Compared to the RdRPs of other Flaviviridae representatives such as the NS5 of the Japanese encephalitis virus (JEV) and dengue virus (DENV) in the Flavivirus genus and the NS5B of the hepatitis C virus (HCV) of the Hepacivirus genus, the pestivirus NS5B contains a unique ∼90-residue N-terminal domain (NTD) that does not have notable sequence homology to any other viral or host proteins. The global conformation of our CSFV NS5B structures is consistent with the recently reported CSFV structure with an RMSD value of 0.9 Å (95% coverage) between the reported structure and our representative C-682 structure. These structures together reveal that the NTD adopts a globular α/β fold with an α-β-α-β-β-α pattern. The NTD interacts with the palm of the RdRP core intra-molecularly with a mixture of hydrophobic and hydrogen bonding interactions. Collectively, these biochemical data indicated that the RNA synthesis fidelity of CSFV NS5B is fine-tuned by its NTD through the intra-molecular interactions with the RdRP palm.

To better understand the nature of the NTD–RdRP intra-molecular interface interactions and whether they regulate the RdRP fidelity, we designed point mutations at the Y471 and E472 sites in the context of the WT NS5B and the N- and C-terminal deletion mutants. Crystallization screenings were performed for all the NTD containing mutant constructs and four of them were successfully crystallized with one construct crystallized under two different conditions. Among these five structures, three of them (Y471A and two forms of C-672_Y471A) maintain the WT conformation with the NTD–RdRP intra-molecular interface maintained. The NTD–RdRP intra-molecular interactions are fully disrupted, and the NTD is rather involved in a non-intensive three-way interaction involving two symmetry-related neighboring NS5B molecules in the crystal lattice. These structural data together suggest that the selection of Y471-E472 mutation sites is valid in perturbing the NTD–RdRP interface, but the interface may not necessarily be fully disrupted by some of the mutations. The effect of E472A mutation was highly consistent with AA mutation (compare lanes 4/8/14/18 to 5/9/15/19), while the effect of Y471A mutation was slightly smaller than that of the E472A and AA mutations (compare lanes 3/7/13/17 to 4/8/14/18 and 5/9/15/19). Although NTD–RdRP disengagement, a situation mimicked by the crystallographic open conformation state in a crystal lattice or the N-91 construct in solution, results in fidelity reduction, engaged NTD–RdRP with perturbation from point mutations can achieve similar level of fidelity reduction.

>MSNWVMQEENKQGNLTPLFEELLQQCPPGGQNKTAHMVSAYQLAQGNWMPTSCHVFMGTISARRTKTHPYEAYVKLRELVEEHKMKTLCPGSSLGKHNDWIIGKIKYQGNLRTKHMLNPGKVAEQLCREGHRHNVYNKTIGSVMTATGIRLEKLPVVRAQTDTTNFHQAIRDKIDKEENLQTPGLHKKLMEVFNALKRPELESSYDAVEWEELERGINRKGAAGFFERKNIGEILDSEKNKVEEIIDNLKKGRNIKYYETAIPKNEKRDVNDDWTAGDFVDEKKPRVIQYPEAKTRLAITKVMYKWVKQKPVVIPGYEGKTPLFQIFDKVKKEWDQFQNPVAVSFDTKAWDTQVTTKDLELIKDIQKYYFKKKWHKFIDTLTMHMTEVPVICADGEVYIRKGQRGSGQPDTSAGNSMLNVLTMVYAFCEATGVPYKSFDRVAKIHVCGDDGFLITERALGEKFASKGVQILAEAGKPQKITEGDKMKVAYQFDDIEFCSHTPIQVRWSDNTSSYMPGRNTTTILAKMATRLDSSGERGTIAYEKAVAFSFLLMYSWNPLIRRICLLVLSTELQVKPGKSTTYYYEGDPISAYKEVIGHNLFDLKRTSFEKLAKLNLSMSVLGAWTRHTSKRLLQDCVNMGVKEGNWLVNADRLVSSKTGNRYIPGEGHTLQGRGSSSHHHHHH[2x]> MEEIYAKFVSQKISKTRWRPLPPGSLQTAETFATGSWDNEENYISLWSIGDFGNLDSDGGFEGDHQLLCDIRHHGDVMDLQFFDQERIVAASSTGCVTVFLHHPNNQTLSVNQQWTTAHYHTGPGSPSYSSAPCTGVVCNNPEIVTVGEDGRINLFRADHKEAVRTIDNADSSTLHAVTFLRTPEILTVNSIGQLKIWDFRQQGNEPSQILSLTGDRVPLHCVDRHPNQQHVVATGGQDGMLSIWDVRQGTMPVSLLKAHEAEMWEVHFHPSNP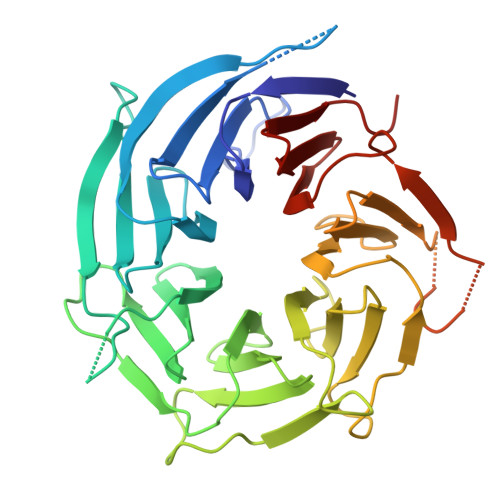EHLFTCSEDGSLWHWDASTDVPEKSSLFHQGGRSSTFLSHSISNQANVHQSVISSWLSTDPAKDRIEITSLLPSRSLSVNTLDVLGPCLVCGTDAEAIYVTRHLFS> ETGSVSKTEHAEINIFSVASGHLYERMLNIMMASVMHHTNHTVKFWFIEQFLSPSFKDFIPHMAAEYGFKYEMVTYKWPHWLRQQKEKQREIWGYKILFLDVL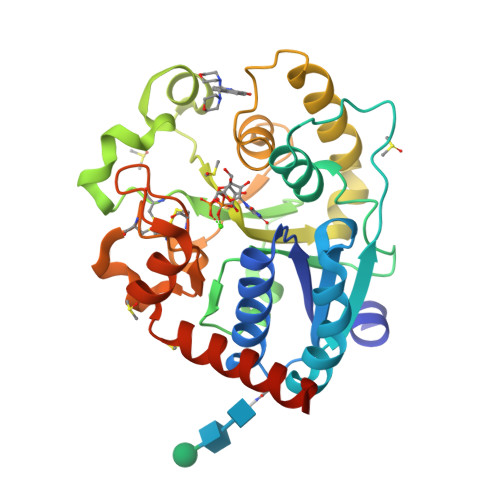FPLSLDKVIFVDADQIVRTDMYDLVEHPLDGAPYGFAPMCDSRVEMEGYRFWKTGYWANYLKGKPYHISALYVVDLQRFRELAAGDRLRQQYHALSADPNSLANLDQDLPNHMQFTIPIATLPQEWLWCETWCSDETLKDARTIDLCNNPMTKEPKLDRARRQVPEWTKYDEEIAELARRVREGTKHHHHHH>[3x]MDHYLVPYNQRANHSKPIPPFLLDLDSQSVPDALKKQTN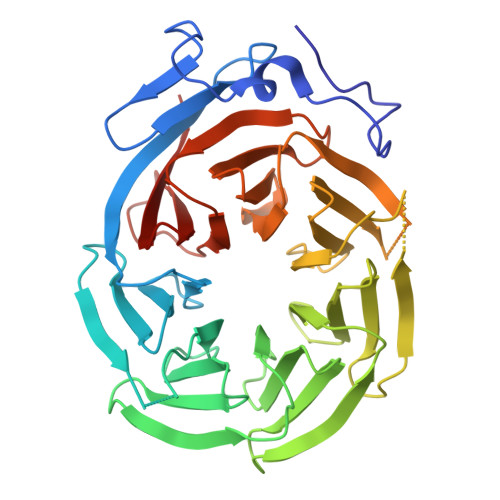DYYILYNPALPREIDVELHKSLDHTSVVCCVKFSNDGEYLATGCNKTTQVYRVSDGSLVARLSDDSAANKDPENLNTSSSPSSDLYIRSVCFSPDGKFLATGAEDRLIRIWDIENRKIVMILQGHEQDIYSLDYFPSGDKLVSGSGDRTVRIWDLRTGQCSLTLSIEDGVTTVAVSPGDGKYIAAGSLDRAVRVWDSETGFLVERLDSENESGTGHKDSVYSVVFTRDGQSVVSGSLDRSVKLWNLQNANNKSDSKTPNSGTCEVTYIGHKDFVLSVATTQNDEYILSGSKDRGVLFWDKKSGNPLLMLQGHRNSVISVAVANGSSLGPEYNVFATGSGDCKARIWKYKKIAPN> MANVDEAILKRVKGWAPYVDAKLGFRNHWYPVMFS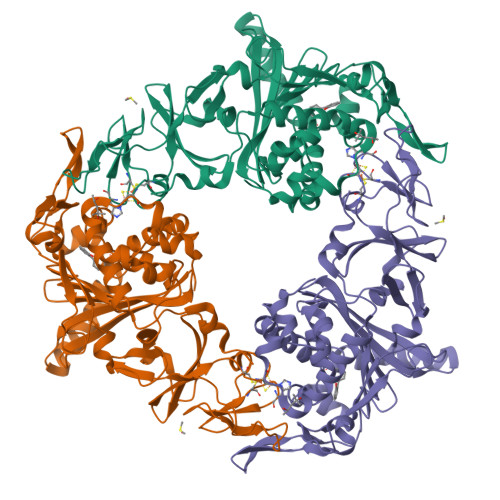KEINEGEPKTLKLLGENLLVNRIDGKLYCLKDRCLHRGVQLSVKVECKTKSTITCWYHAWTYRWEDGVLCDILTNPTSAQIGRQKLKTYPVQEAKGCVFIYLGDGDPPPLARDTPPNFLDDDMEILGKNQIIKSNWRLAVENGFDPSHIYIHKDSILVKDNDLALPLGFAPGGDRKQQTRVVDDDVVGRKGVYDLIGEHGVPVFEGTIGGEVVREGAYGEKIVANDISIWLPGVLKVNPFPNPDMMQFEWYVPIDENTHYYFQTLGKPCANDEERKKYEQEFESKWKPMALEGFNNDDIWAREAMVDFYADDKGWVNEILFESDEAIVAWRKLASEHNQGIQTQAHVSGLEHHHHHH>SNAMSKLPENFLWGGAVAAHQLEGGWQEGGKGISVADVMTAGRHGVAREITAGVLEGKYYPNHEAIDFYHHYKEDVKLFAEMGFKCFRTSIAWTRIFPKGDEAEPNEAGLQFYDDLFDECLKYGIEPVVTLSHFELPYHLVTEYGGFTNRKVIDFFVHFAEVCFRRYKDKVKYWMTFNEINNQANYQEDFAPFTNSGIVYKEGDDREAIMYQAAHYELVASARAVKIGHAINPNLNIGCMVAMCPIYPATCNPKDILMA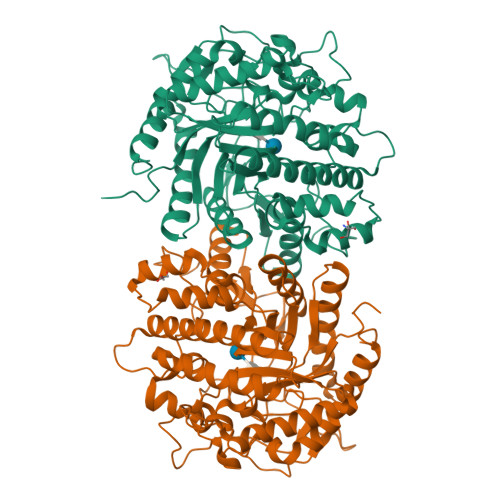QKAMQKRYYFADVHVHGFYPEHIFKYWERKAIKVDFTERDKKDLFEGTVDYIGFSYYMSFVIDAHRENNPYYDYLETEDLVKNPYVKASDWDWQIDPQGLRYALNWFTDMYHLPLFIVQNGFGAIDQVEADGMVHDDYRIDYLGAHIKEMIKAVDEDGVELMGYTPWGCIDLVSAGTGEMRKRYGFIYVDKDDEGKGTLKRSPKLSFNWYKEVIASNGDDI[2x]Certain bacterial species from genera such as Paracoccus, Pseudomonas, and Alcaligenes have evolved to use DMF as a sole carbon and nitrogen source for growth via degradation by a dimethylformamidase (DMFase). We show that DMFase from Paracoccus sp. strain DMF is a halophilic and thermostable enzyme comprising a multimeric complex of the α2β2 or (α2β2)2 type. The active site consists of a mononuclear iron coordinated by two Tyr side‐chain phenolates and one carboxylate from Glu. The Fe3+ ion in the active site catalyzes the hydrolytic cleavage of the amide bond in DMF.

When the purified native or recombinant parDMFase was imaged on ice by electron cryo‐microscopy (cryoEM), the micrographs unambiguously revealed two populations: a smaller molecule measuring approximately 100 Å diameter and a larger structure of approximately 150 Å in diameter could be identified. Subsequent 2D classification showed that the smaller unit was a dimer, and the larger structure was a dimer of dimers. The dimer of the parDMFase is made of two α and two β subunits with a total mass of 200 kDa. In the presence of low salt, the enzyme is predominantly in the dimeric form, and this equilibrium shifted to the tetramer at higher salt concentrations (≥200 mm). Subsequently, we collected two data sets with no salt and 200 mm NaCl yielding reconstructions with an overall resolution of 3 Å (dimer) and 2.8 Å (tetramer), respectively. The high quality of the maps allowed de novo tracing of polypeptide chains of both the large and small subunits. We used the dimer map for the initial tracing, and the final model is shown in Figure 2 B. The model from the dimer was used to obtain the tetramer model. The initial EM map clearly showed a large density around residues Y440, Y399, and E521 that could not be accounted for by amino acids. The mononuclear Fe atom is tetra‐coordinated with the protein. It is coordinated to two phenolates of tyrosine residues (Y399 and Y440 serve as monodentate ligands), and a glutamic acid carboxylate side chain (E521 serves as a bidentate ligand).

>[2x]MKDIAIRGYCDRPSVATGETIRFYVSANETRGTFDAELVRLIHGDSNPAGPGYKEEAIKSDLEGQYPARFQRTQFGSYVEVADPDAGLQPDGAFSVHLFLWSTTPSRGRQGIASRWNDERQSGWNLAIEDGRVVFTIGDGSGATSSVVSDRPLFQQIWYSITGVYDPEKKQLRLYQKSVVNRTNSRFGLVVPLDSDCAVSADATVKAADSETSLLIAGLGEAAAQDGRTWCIAHYNGKVDAPKIYGCALGQDDAEKLSRGEIVRPISRLAHWDFSAGIGLNGIPTDHVVDASGYGHHGRCMNQPSRGSTGWNWDGHEENFIHCPEQYGALWFHEDCLDDCRWEKDFEFTVPEGLKSDFYAVKIRYEDTEDYIPFFVLPPRGTATAPILVIASTLSYLAYANEQIMHKADIGQAVAGHTPVLNENDVELHKNLSYYGLSTYDGHIDGRGVQYTSWRRPIMNLRPKHRQGFGSIWELPADLHLIDWLNHNGFEYDVATEHDLNDQGAELLRRYKVVLTGSHPEYQTWANADAWEDYLADGGRGMYLAANGMYWIVEVHPEKPWVMEVRKELGVTAWEAPPGEYHYSTNGRRGGRFRGRARATQKIWGTGMSSFGFDHSGYFVQMPDSQDERVAWIMEGIDPEERIGDGGLVGGGAGGYELDRYDLALGTPPNTLLLASSVEHSVVYTVIPDDKAFPHPGMNGGEHPFVRADITYFSTANGGGMFATSSISWLGSLSWNDYDNNVSKMTKNVLNQFIKDEPAPRVKLAAALEHHHHHH;>MTEASESCVRDPSNYRDRSADWYAFYDERRRKEIIDIIDEHPEIVEEHAANPFGYRKHPSPYLQRVHNYFRMQPTFGRYYIYSEREWDAYRIATIREFGELPELGDERFKTEEEAMHAVFLRRIEDVRAELA[2x]> MLGLKTSIIGRRVIYFQEITSTNEFAKTSYLEEGTVIVADKQTMGHGALNRKWESPEGGLWLSIVLSPKVPQKDLPKIVFLGAVGVVETLKEFSIDGRIKWPNDVLVNYKAIAGVLVEGKGDKIVLGIGLNV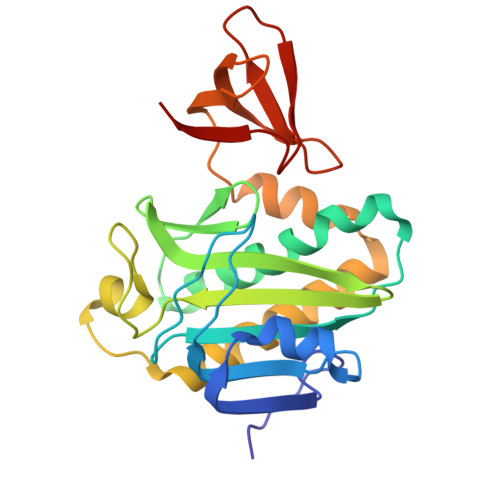NNKVPNGATSMKLELGSEVPLLSVFRSLITNLDRLYLNFLKNPMDILNLVRDNMILGVRVKILGDGSFEGIAEDIDDFGRLIIRLDSGEVKKVIYGDVSLRFL> MHHHHHHHHVEAAPTAQQQLLEQVRLGEATHREDLVQQSLYRLELIDPNNPDVVAARFRSLLRQGDIDGAQKQLDRLSQLAPSSNAYKSSRTTMLLSTPDGRQALQQARLQATTGHAEEAVASYNKLFNGAPPEGDIAVEYWSTVAKIPARRGEAINQLKRINADAPGNTGLQNNLALLLFSSDRRDEGFAVLEQMAKSNAGREGASKIWYGQIKDMPVSDASVSALKKYLSIFSDGDSVAAAQSQLAEQQKQLADPAFRARAQGLAAVDSGMAGKAIPELQQAVRANPKDSEALGALGQAYSQKGDRANAVANLEKALALDPHSSNNDKWNSLLKVNRYWLAIQQGDAALKANNPDRAERLFQQARNVDNTDSYAVLGLGDVAMARKDYPAAERYYQQTLRMDSGNTNAVRGLANIYRQQSPEKAEAFIASLSASQRRSIDDIERSLQNDRLAQQAEALENQGKWAQAAALQRQRLALDPGSVWITYRLSQDLWQAGQRSQADTLMRNLAQQKSNDPEQVYAYGLYLSGHDQDRAALAHINSLPRAQWNSNIQELVNRLQSDQVLETANRLRESGKEAEAEAMLRQQPPSTRIDLTLADWAQQRRDYTAARAAYQNVLTREPANADAILGLTEVDIAAGDKAAARSQLAKLPATDNASLNTQRRVALAQAQLGDTAAAQRTFNKLIPQAKSQPPSMESAMVLRDGAKFEAQAGDPTQALETYKDAMVASGVTTTRPQDNDTFTRLTRNDEKDDWLKRGVRSDAADLYRQQDLNVTLEHDYWGSSGTGGYSDLKAHTTMLQVDAPYSDGRMFFRSDFVNMNVGSFSTNADGKWD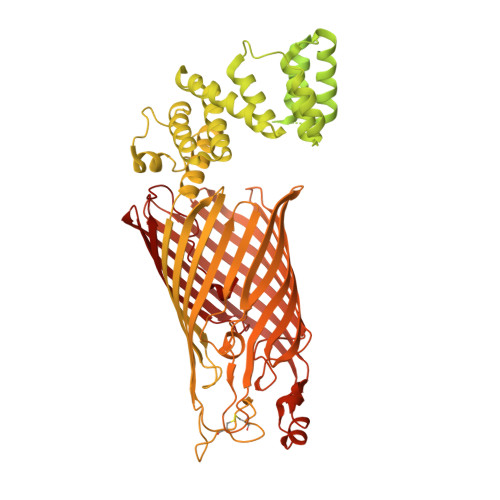DNWGTCTLQDCSGNRSQSDSGASVAVGWRNDVWSWDIGTTPMGFNVVDVVGGISYSDDIGPLGYTVNAHRRPISSSLLAFGGQKDSPSNTGKKWGGVRADGVGLSLSYDKGEANGVWASLSGDQLTGKNVEDNWRVRWMTGYYYKVINQNNRRVTIGLNNMIWHYDKDLSGYSLGQGGYYSPQEYLSFAIPVMWRERTENWSWELGASGSWSHSRTKTMPRYPLMNLIPTDWQEEAARQSNDGGSSQGFGYTARALLERRVTSNWFVGTAIDIQQAKDYAPSHFLLYVRYSAAGWQGDMDLPPQPLIPYADW>MLYKLLNVLWLVAVSNAIPGTPVIDWADRNYALVEINYEATAYENLIKPKEQVDVQVSWNVWNGDIGDIAYVLFDEQQVWKGDAESKRATIKVLVSGQFNMRVKLCNEDGCSVSDPVLVKVADTDGGHLAPLEYTWLENNKPGRREDKIVAAYFVEWGVYGRNFPVDKVPLPNLSHLLYGFIPICGGDGINDALKTISGSFESLQRSCKGREDFKVAIHDPWAAVQKPQKSVSAWNEPYKGNFGQLMAAKLANPHLKILPSIGGWTLSDPFYFMHDVEKRNVFVDSVKEFLQVWKFFDGVDVDWEFPGGKGANPSLGDAERDAKTYILLLEELRAMLDDLEAQTGRVYELTSAISAGYDKIAVVNYAEAQKSLGKIFLMSYDFKGAWSNTDLGYQTTVYAPSWNSEELYTTHYAVDALLKQGVDPNKIIVGVAMYGRGWTGVTNYTNDNYFSGTGNGPVSGTWEDGVVDYRQIQKDLNNYVYTFDSAAQASYVFDKSKGDLISFDSVDSVLGKVKYVDRNKLGGLFAWEIDADNGDLLNAINAQFKPKDEL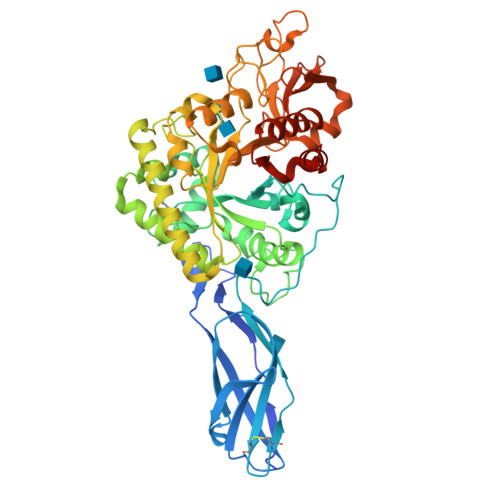[2x]> GFKTFYIKVILKEGTQLKSARIYLVFHKLEELKCEVVRTIPSVEEIEEEKFENEVELFVISPVDLEKLSEALSSIADIERVIIKEV;> GKRVLIVDDAAFMRMMLKDIITKAGYEV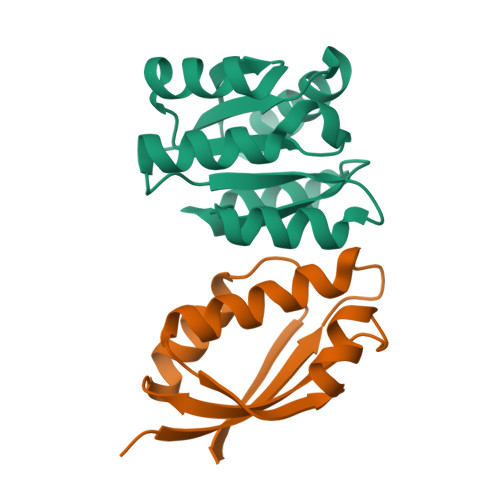AGEATNGREAVEKYKELKPDIVTMDITMPEMNGIDAIKEIMKIDPNAKIIVCSAMGQQAMVIEAIKAGAKDFIVKPFQPSRVVEALNKVS> APMTEVEQKAAAGVFDDANVRDRALTDWDGMWQSVY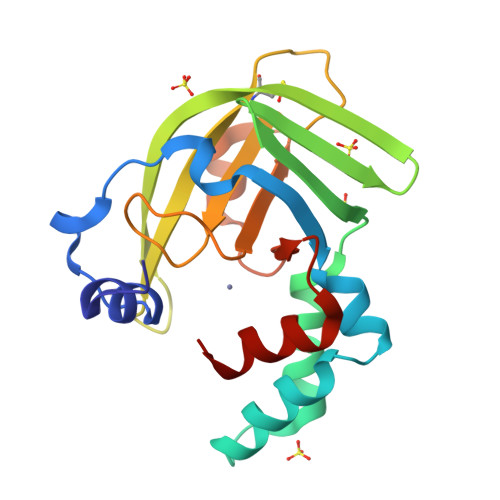PYLVSGELDPVFRQKAKKDPEKTFEDIKAYYRKGYVTNVETIGIENGVIEFHRDNNVASCKYNYAGYKILTYASGKKGVRYLFECKDANSKAPKYVQFSDHIIAPRKSAHFHIFMGNTSQQALLQEMENWPTYYPYQLKANEVVDEMLHH>AIAMTHPDISVDVLVIGAGPTGLGAAKRLNQIDGPSWMIVDSNETPGGLASTDVTPEGFLYDVGGHVIFSHYKYFDDCLDEALPKEDDWYTHQRISYVRCQGQWVPYPFQNNISMLPKEEQVKCIDGMIDAALEARVANTKPKTFDEWIVRMMGTGIADLFMRPYNFKVWAVPTTKMQCAWLGERVAAPNLKAVTTNVILGKTAGNWGPNATFRFPARGGTGGI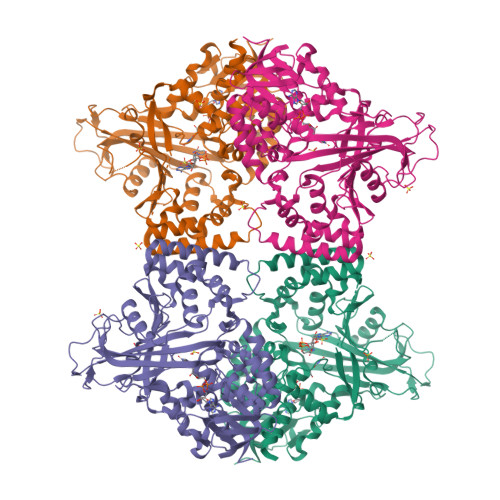WIAVANTLPKEKTRFGEKGKVTKVNANNKTVTLQDGTTIGYKKLVSTMAVDFLAEAMNDQELVGLTKQLFYSSTHVIGVGVRGSRPERIGDKCWLYFPEDNCPFYRATIFSNYSPYNQPEASAALPTMQLADGSRPQSTEAKEGPYWSIMLEVSESSMKPVNQETILADCIQGLVNTEMLKPTDEIVSTYHRRFDHGYPTPTLEREGTLTQILPKLQDKDIWSRGRFGSWRYEVGNQDHSFMLGVEAVDNIVNGAVELTLNYPDFVNGRQNTERRLVDGAQVFAKSKAQ[4x]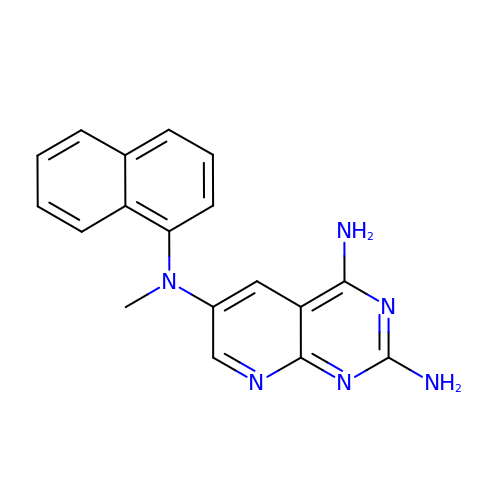N~6~-methyl-N~6~-(naphthalen-1-yl)pyrido[2,3-d]pyrimidine-2,4,6-triamine | C18 H16 N6 | QNASXWBMQABDSW-UHFFFAOYSA-N> MSSMILTQFGPFIESISGITDQSNDVFEDAAKAFSMFTRSDVYKALDEIPFSDDAMLPIPPTIYTKPSH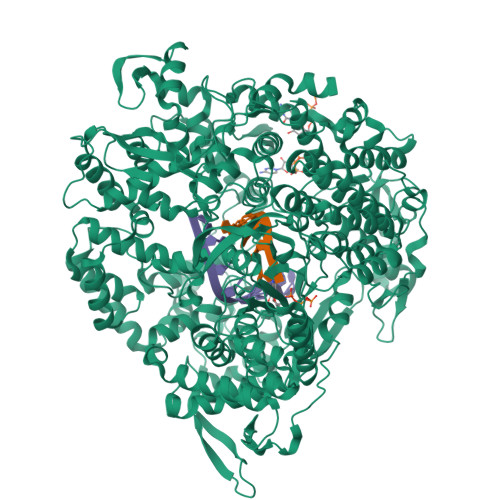DSYYYIDALNRVRRKTYQGPDDVYVPNCSIVELLEPHETLTSYGRLSEAIENRAKDGDSQARIATTYGRIAESQARQIKAPLEKFVLALLVAEAGGSLYDPVLQKYDEIPDLSHNCPLWCFREICRHISGPLPDRAPYLYLSAGVFWLMSPRMTSAIPPLLSDLVNLAILQQTAGLDPSLVKLGVQICLHAAASSSYSWFILKTKSIFPQNTLHSMYESLEGGYCPNLEWLEPRSDYKFMYMGVMPLSAKYARSAPSNDKKARELGEKYGLSSVVGELRKRTKTYVKHDFASVRYIRDAMACTSGIFLVRTPTETVLQEYTQSPEIKVPIPQKDWTGPIGEIRILKDTTSSIARYLYRTWYLAAARMAAQPRTWDPLFQAIMRSQYVTARGGSGAALRESLYAINVSLPDFKGLPVKAATKIFQAAQLANLPFSHTSVAILADTSMGLRNQVQRRPRSIMPLNVPQQQVSAPHTLTADYINYHMNLSPTSGSAVIEKVIPLGVYASSPPNQSINIDISACDASITWDFFLSVIMAAIHEGVASSSIGKPFMGVPASIVNDESVVGVRAARPISGMQNMIQHLSKLYKRGFSYRVNDSFSPGNDFTHMTTTFPSGSTATSTEHTANNSTMMETFLTVWGPEHTDDPDVLRLMKSLTIQRNYVCQGDDGLMIIDGTTAGKVNSETIQNDLELISKYGEEFGWKYDIAYDGTAEYLKLYFIFGCRIPNLSRHPIVGKERANSSAEEPWPAILDQIMGVFFNGVHDGLQWQRWIRYSWALCCAFSRQRTMIGESVGYLQYPMWSFVYWGLPLVKAFGSDPWIFSWYMPTGDLGMYSWISLIRPLMTRWMVANGYVTDRCSTVFGNADYRRCFNELKLYQGYYMAQLPRNPKKSGRAASREVREQFTQALSDYLMQNPELKSRVLRGRSEWEKYGAGIIHNPPSLFDVPHKWYQGAQEAAIATREELAEMDETLMRARRHSYSSFSKLLEAYLLVKWRMCEAREPSVDLRLPLCAGIDPLNSDPFLKMVSVGPMLQSTRKYFAQTLFMAKTVSGLDVNAIDSALLRLRTLGADKKALTAQLLMVGLQESEADALAGKIMLQDVNTVQLARVVNLAVPDTWMSLDFDSMFKHHVKLLPKDGRHLNTDIPPRMGWLRAILRFLGAGMVMTATGVAVDIYLEDIHGGGRSLGQRFMTWMRQEGRSA> SSTFSASDFNSERYSSSRPSYPSDFYKMIDEYHDGERKLLVDVGCGPGTATLQMAQELKPFEQIIGSDLSATMIKTAEVIKEGSPDTYKNVSFKISSSDDFKFLGADSVDKQKIDMITAVECAHWFDFEKFQRSAYANLRKDGTIAIWGYADPIFPDYPEFD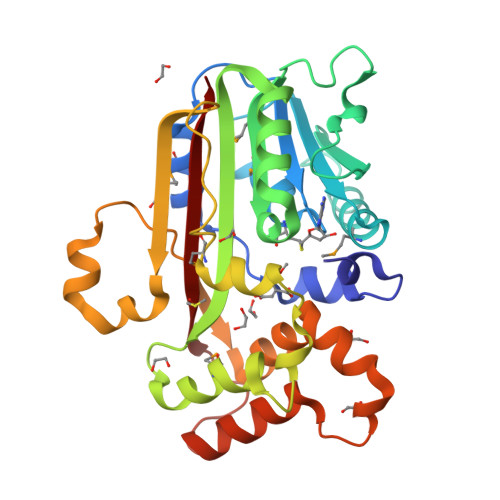DLMIEVPYGKQGLGPYWEQPGRSRLRNMLKDSHLDPELFHDIQVSYFCAEDVRDKVKLHQHTKKPLLIRKQVTLVEFADYVRTWSAYHQWKQDPKNKDKEDVADWFIKESLRRRPELSTNTKIEVVWNTFYKLGKRV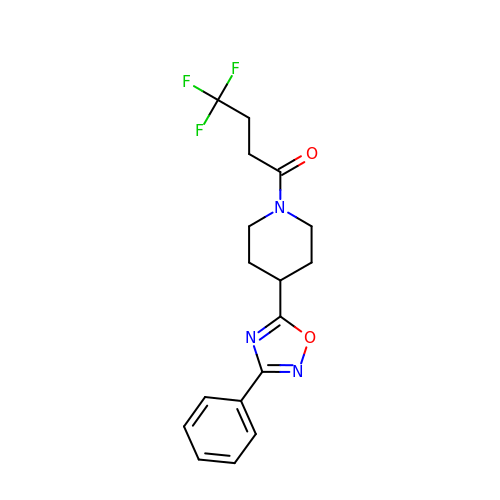4,4,4-tris(fluoranyl)-1-[4-(3-phenyl-1,2,4-oxadiazol-5-yl)piperidin-1-yl]butan-1-one | C17 H18 F3 N3 O2 | ROEPMLPFAFHQCH-UHFFFAOYSA-N> GAMAMSDLPIEFTELVDLMSLGISPQFLDFRSTTFESDHFVTVRETKDGTNSVAIVDLAKGNEVTRKNMGGDSAIMHPSQMVISVRANGTIVQIFNLETKSKLKSFTLDEPVIFWRWLSETTLGFVTARSILTSNVFDGNVNAKPQLLTLRHANLNNTQIINFVANKNLDWFAVVGILQENGRIAGRIQLFSKQRNISQAIDGHVAIFTNILLEGNGSTPVQVFVTGNRNATTGAGELRIIEIDHDASLPSQYQKETTDIFFPPDATNDFPIAVQVSEKYGIIYLLTKYGFIH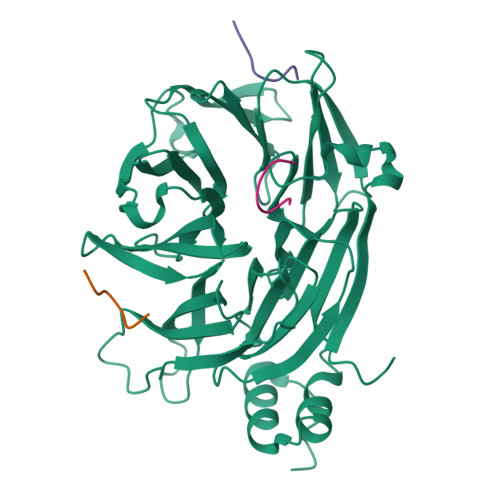LYELETGTNLFVNRITAESVFTAAPYNHENGIACINKKGQVLAVEISTSQIVPYILNKLSNVALALIVATRGGLPGADDL;>GYTLIDL[3x]>MSGILALGAYVPERVMTNADFEAYLDTSDEWIVTRTGIKERRVAAEDEYTSDLAFKAVEDLLRRHPGALEGVDAVIVATNTPDALFPDTAALVQARFGLKAFAYDLLAGCPGWIYALAQAHALVEAGLAQKVLAVGAEALSKIIDWNDRATAVLFGDGGGAAVVGKVREGYGFRSFVLGADGTGAKELYHACVAPRLPDGTSMKNRLYMNGREVFKFAVRVMNTATLEAIEKAGLTPEDIRLFVPHQANLRIIDAARERLGLPWERVAVNVDRYGNTSTASIPLALKEAVDAGRIREGDHVLLVSFGAGLTWAAAVLTW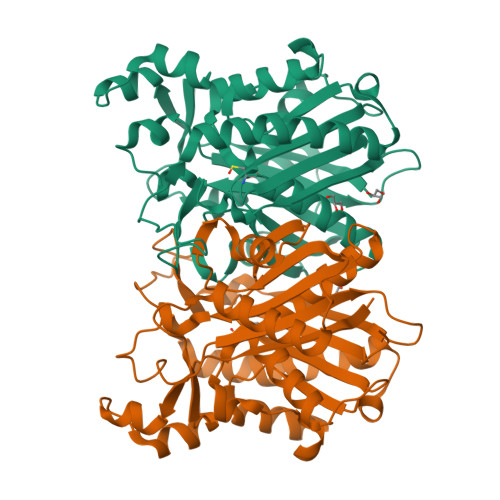GGA[4x]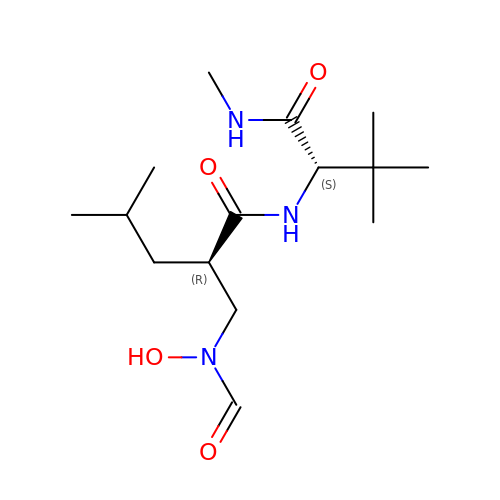N~2~-[(2R)-2-{[formyl(hydroxy)amino]methyl}-4-methylpentanoyl]-N,3-dimethyl-L-valinamide | C15 H29 N3 O4 | YRLGSCVOSAUJJE-VXGBXAGGSA-N>[2x]MGSSHHHHHHSSGENLYFQGHMAENIPFSPQPPEIHAGSWVLMDYTTGQILTAGNEHQQRNPASLTKLMTGYVVDRAIDSHRITPDDIVTVGRDAWA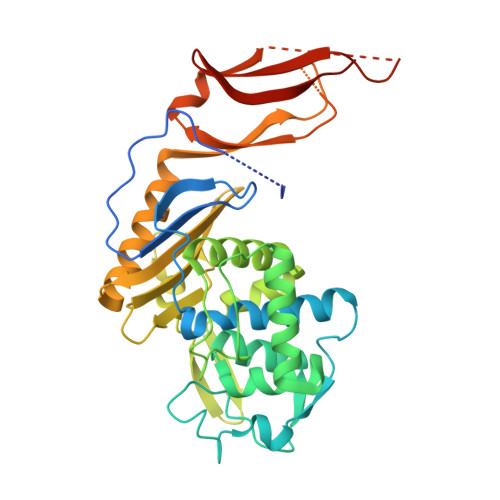KDNPVFVGSSLMFLKEGDRVSVRDLSRGLIVDSGNDACVALADYIAGGQRQFVEMMNNYAEKLHLKDTHFETVHGLDAPGQHSSAYDLAVLSRAIIHGEPEFYHMYSEKSLTWNGITQQNRNGLLWDKTMNVDGLKTGHTSGAGFNLIASAVDGQRRLIAVVMGADSAKGREEEARKLLRWGQQNFTTVQILHRGKKVGTERIWYGDKENIDLGTEQEFWMVLPKAEIPHIKAKYTLDGKELTAPISAHQRVGEIELYDRDKQVAHWPLVTLESVGEG>[5x]MGFWGLEVKPGKPQAYNPKNEQGKIHVTQATLGT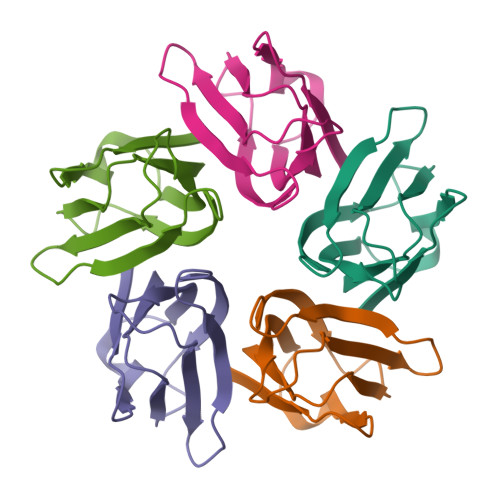GLSKEKSVIQCSIGDKAPIALCSLLPNKIECCPLNLEFDDDDEPVEFTVTGDRSIHLSGFLEYYQDLEHHHHHH> ARVTVQDAVEKIGNRFDLVLVAARRARQMQVGGKDPLVPEENDKTTVIALREIEEGLINNQILDVRERQEQQEQEAAEL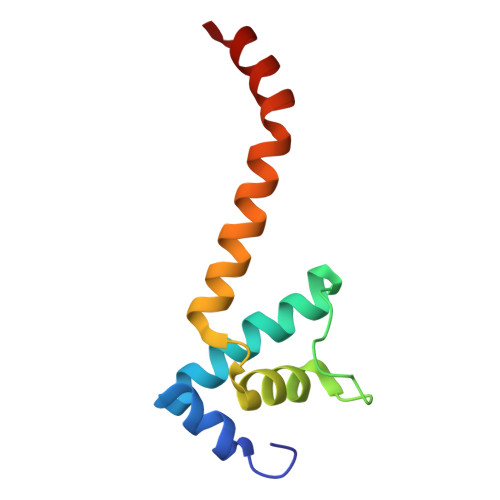QAVTAIAEGRR>GSHMGGIEVLAVRTGPDSITEIEAYLNPRMGQPQNEDFYGFSDNVTVSDDFGSDAPPWKQFPCYSTARISLPMLNQDMTSDTILMWEAISCRTEVMGVNMLTNVHSAQKRVYENDREGTGIGVEGMGYHMFAIGGEPLELQFMVFNHRATYPAEATVIKNPGASSQVFDPNLKGTLTADGVFPVEAWGPDPFKNENTRYFGQYTGGTQTPPVLTFTNTQTTILLDENGVGPLCKGDGLFLSCADIVGFFTQHNKKMSFRGLPRYFRVTLR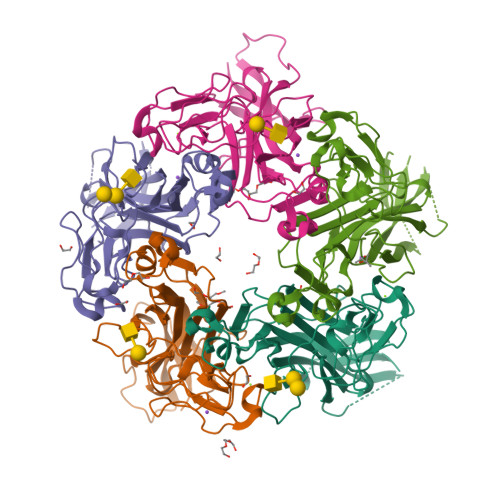KRVVKN[10x]>[2x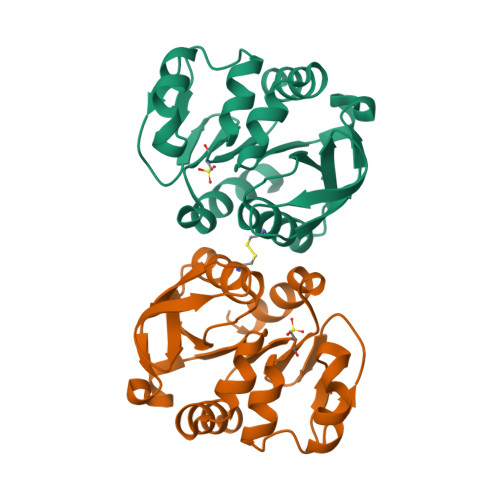]MKVLFLSADGFEDLELICPLHRIKEEGHEVYVASFERGKITGKHGYSVNVDLAFEEVGPDEFDALVLPGGRAPEIVRLNEKAIEITRKMFEAGKPVASICHGPQILISAGVLKGRKGTSTITIRDDVVNAGAEWVNEEVVVDGNWVSSRHPGDLYAWMREFVKLLK>MEHKRGHVLAVPYPAQGHITPFRQFCKRLHFKGLKTTLALTTFVFNSINPDLSGPISIATISDGYDHGGFETADSIDDYLKDFKTSGSKTIADIIQKHQTSDNPITCIVYDAFLPWALDVAREFGLVATPFFTQPCAVNYVYYLSYINNGSLQLPIEELPFLELQDLPSFFSVSGSYPAYFEMVLQQFINFEKADFVLVNSFQELELHENELWSKACPVLTIGPTIPSIYLDQRIKSDTGYDLNLFESKDDSFCINWLDTRPQGSVVYVAFGSMAQLTNVQMEELASAVSNFSFLWVVRSSEEEKLPSGFLETVNKEKSLVLKWSPQLQVLSNKAIGCFLTHCGWNSTMEALTFGVPMVAMPQWTDQPMNAKYIQDVWKAGVRVKTEKESGIAKREEIEFSIKEVMEGERSKEMKKNVKKWRDLAVKSLNEGGSTDTNIDTFVSRVQSK[2x]

UGT74F1 and UGT74F2 are the enzymes responsible for the in vivo glucosylation of SA in A. thaliana. In UGT74F1, glucose is transferred to the hydroxyl of SA, creating a glucoside; in UGT74F2, glucose is transferred to the carboxylate group of SA to create a glucose ester. UGT74F2 exhibits the GT-B fold with ligands bound in the cleft between the two domains –the N-terminal domain is comprised of residues 1–245, while 246–449 make up the C-terminal domain. UDP and SA interact primarily with residues in the C- and N-terminal domain, respectively.

We crystalized UGT74F2T15S and UGT74F2T15A in complex with UDP and SA or UDP and 2-BA. As the findings with both mutants were identical, we will present further the structures of UGT74F2T15S. In contrast, UGT74F2T15A and UGT74F2T15S form both SGE and SAG; UGT74F2T15A has wild-type activity for SGE formation, better than UGT74F2T15S, and both mutants form about 5-fold more SAG than the wild-type. Relative to the wild-type enzyme, mutation of residue 15 to serine or alanine in UGT74F2 did not lessen the specific activity for SGE formation, but did increase the formation of SAG. Altogether, these data suggest that the structure of residue 15 is important for SAG formation in both UGT74F1 and UGT74F2: the smaller the side-chain, the higher SAG formation (with Ala > Ser > Thr). Perhaps the presence of a branched amino acid at residue 15 constrains SA binding in a particular conformation and functions in organizing the binding pocket.> GTGMDAGKKDVYILSAVRTPIASFRSTLTSLSAVDLGIVVTKEAIKRSLLPSSAIEETIVGNVLSAGLGQNIARQISIASEIPKSSQCVTINKVCSSSMKAIIMGAQAIQVGYRRIVVALGSESMSNAPFYVPRGEIPFGGVQLVDALQRDGLMDSIEYQPMGLCAEKTVKDYAFTREQLDAYAIESYRKAEHAWKEGAFNKEVVPVSVPQKRGSKVVLTEDEEYKRLIPEKVPALHPAFLKDGSGTITAANASTINDGAAACVLASGEVVQEGRLKPIAKVLSYAEAGVEPIDFTVAPALAVKQLLSQSGLDEESIALWEINEAFSVTGLAFIKELRLDPKRVNVRGGAVALGHPLGASGARIVVTLVHALKSDELGVAAICNGGGEASA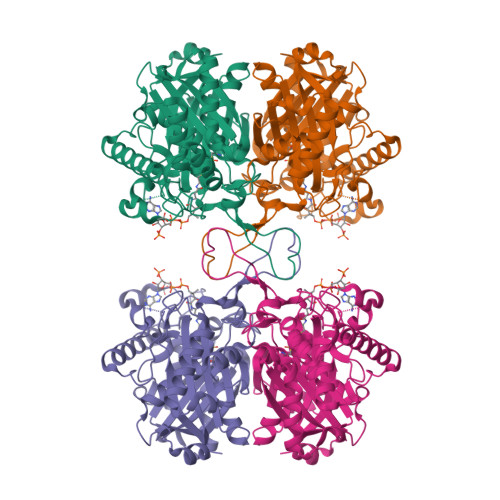ILIKKL Eukaryotes possess eight highly conserved Lsm (like Sm) proteins that assemble into circular, heteroheptameric complexes, bind RNA, and direct a diverse range of biological processes. Among the many essential functions of Lsm proteins, the cytoplasmic Lsm1–7 complex initiates mRNA decay, while the nuclear Lsm2–8 complex acts as a chaperone for U6 spliceosomal RNA. The Sm family includes the Sm, Lsm (“Like Sm”), and bacterial Hfq proteins. These proteins share a conserved “Sm fold” consisting of an amino-terminal alpha helix followed by five antiparallel beta strands that form small beta barrels that assemble into ring-shaped hexamers or heptamers. Here, we elucidate the molecular basis for Lsm-RNA recognition and present four high-resolution structures of Lsm complexes bound to RNAs.

Since deletion of the carboxyl terminus of Lsm1 generally enhances binding affinity, we therefore crystallized the Lsm1Δ56C–7 variant of the Lsm1–7 complex bound to the U-tract RNAs UUUUUA and AUUUUG and determined their structures to resolutions of 1.8 and 2.1 Å, respectively. In the structure of Lsm1Δ56C–7 bound to AUUUUG, all nucleotides are visible within the electron density map. The path of the RNA around the interior of the Lsm1–7 torus is a right-handed helix, with the phosphodiester backbone in the center and the nucleobases splayed out into binding pockets. The six nucleotides of the RNA make an almost complete turn with the last nucleotides 6 Å below the first. The 5′ adenosine interacts with the noncanonical binding pocket on Lsm5 by stacking on Tyr39. The 3′ G also interacts with Lsm5 by forming a hydrogen bond to Asn66 in a manner that is similar to the interaction observed for the terminal adenine of UUUUUA, except the asparagine side chain donates a hydrogen bond to the guanine oxygen instead of an adenine nitrogen. The structures explain why oligonucleotides harboring these sequences bind with nearly identical affinities to Lsm1Δ56C–7. In the crystal structures, the 5′ end of the RNA hexamer is nearest the “proximal face” of Lsm1–7 while the 3′ end is nearest the “distal face”, the same orientation as in the Sm ring where the bound RNA passes completely through the center of the torus. Lsm1–7 binds tightly to the sequence AUUUUR, and this sequence is highly reminiscent of sequences found in 3′-UTR regions that undergo adenine/uridine-rich element (ARE) mRNA decay.

> GSMNQATQIIPFTTSGSLVDYVDRKVIVVLRDGKKLIGILRSFDQFANLMLQYTIERIYVDDMYGDIDRGVYIVRGENVVLLGELD;> MLFYSFFKTLIDTEVTVELKNDMSIRGILKSVDQFLNVKLENISVVDASKYPHMAAVKDLFIRGSVVRYVHMSSAYVDTILLADACRRDLANNKRQ;> GSMESAQAVAEPLDLVRLSLDEIVYVKLRGDRELNGRLHAYDEHLNMVLGDAEEIVTIFDDEETDKDKALKTIRKHYEMLFVRGDSVILIAPPRN;> MLPLTLLNATQGRPILVELKNGETFNGHLENCDNYMNLTLREVIRTMPDGDKFFRLPECYIRGNNIKYLRIQDEVLSQVAKQQAQQRENRGSRFRGRGQRGRGNYGHTAPNRRGRGRGGHMWSHPQFEK;> MSMTILPLELIDKCIGSNLWVIMKSEREFAGTLVGFDDYVNIVLKDVTEYDTVTGVTEKHSEMLLNGNGMCMLIPGGKPE;> GSMDSSPNEFLNKVIGKKVLIRLSSGVDYKGILSCLDGYMNLALERTEEYVNGKKTNVYGDAFIRGNNVLYVSALDD;> MSSLQKRPGPGNSSQPTERPRKESILDLSRYQDQRIQATFTGGRQITGILKGFDQLMNLVLDDVEEQLRNPEDGKLTGAIRKLGLVVVRGTTLVLIAPMDGSEEIPNPFVQAE>[2x]STVVTTESGLKYEDLT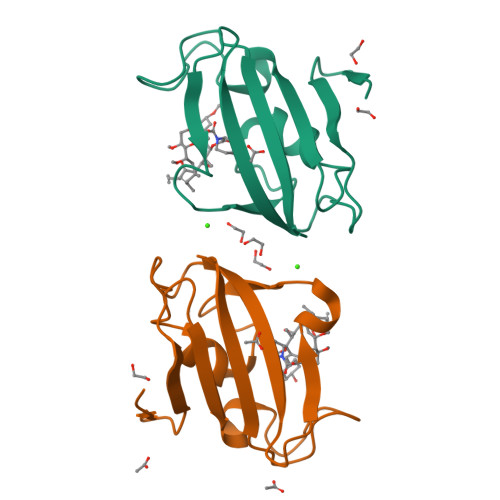EGSGAEARAGQTVSVHYTGWLTDGQKFDSSKDRNDPFAFVLGGGHVIKGWDEGVQGMKVGGVRRLTIPPQLGYGARGAGGVIPPNATLVFEVELLDV>[2x]MAAKVSSDPLVIGRVIGDVVDHFTSTVKMSVIYNSNNSIKHVYNGHELFPSAVTSTPRVEVHGGDMRSFFTLIMTDPDVPGPSDPYLREHLHWIVTDIP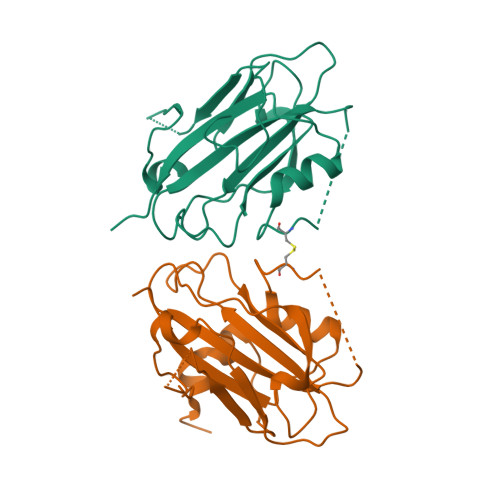GTTDSSFGKEVVSYEMPRPNIGIHRFVFLLFKQKKRGQAMLSPPVVCRDGFNTRKFTQENELGLPVAAVFFNCQRETAARRR>SMRKKIFKPEELRQALMPTLEALYRQDPESLPFRQPVDPQLLGIPDYFDIVKNPMDLSTIKRKLDTGQYQEPWQYVDDVWLMFNNAWLYNRKTSRVYKFC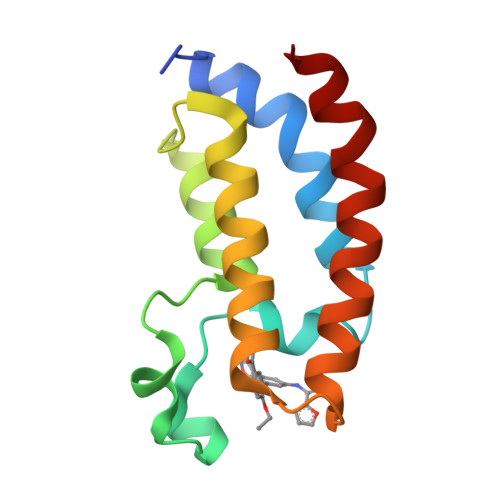SKLAEVFEQEIDPVMQSLG[4x]> MKRARSANIPGAILHSLAELQDGLNAMIDPSWRAVRSLDNWALAITMESTELLDSYPWKWWKNLNATPDLANVRIELVDIFHFSLSGAMQMRSTPDDEIPAASLKPLKEVMTTFLPAKECTSDPYGFVFFPLTDTQNAIASFRNIIQLANAYRFDVIIE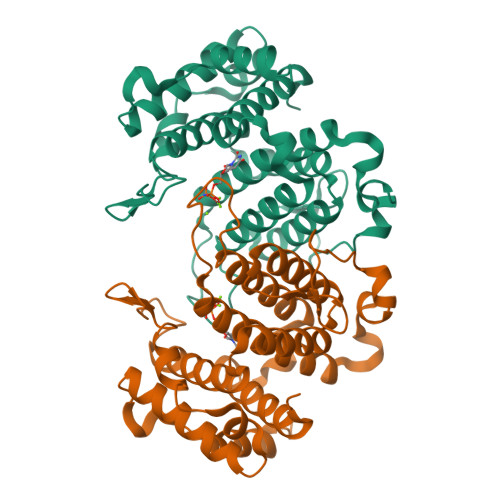CIIYAAEDLGFNLVAYYIAKHTLNCIRQLSGYKDGSYVKVNNGVEDNSLLHNCIKDVSLDEVLDADKYVQAWNSIMANVYEAFQIKESDRKDAERWFALAKENRLAIKA>MGRDPNSTDNIRPTYQTDANGTYPTNSWQVTGQQNVINQRGGDQVSGWDNNTIWNGDATDTTNSYLKFGDPNNPDYQIRKYAKETNTPGLYDVYLNVKGNKQQNVKPVDIVLVVDMSGSMESNRWGTNRAGAVRTGVKNFLTSIQNAGLGNYVNVGLIGFSSPGYIGGKSGYISVKLGKAGNASQQQAINGALSPRFQGGTYTQIGLRQGSAMLNADTSGNKKMMILLTDGVPTFSNEVINSEWINGTLYGTNFGSSRDEPGNTARLRWPYTDSSGHYIYDTWPATLGEAKIAKDSGNEVHALGIQLADDDHYMTKEKIRQNMQLITNSPDLYEDADSADAVEAYLNNQAKDIIKNFNTVTDGTITDPIGTQFQYANNQATVTSVGKQTVPASELPSAAIQDGQLTVNHMNLGQDQEVQIHYQVRIKTEDAGFKPDFWYQMNGETLLTPKAGAAAVDFGIPSGRAPATTVYVQKQWRQLSNQSLPDTLNVTVQRKVADGSLDPNWQQTLVLKKADNWKASFTAPAYNNQGQSFSYVVKSEDASGIDLSSFISSQNMDQQTATLTLTNQQYGFQFQKKTTDGTDLSADQLKAMQFNLTQYSDNSFQQASKTNAITST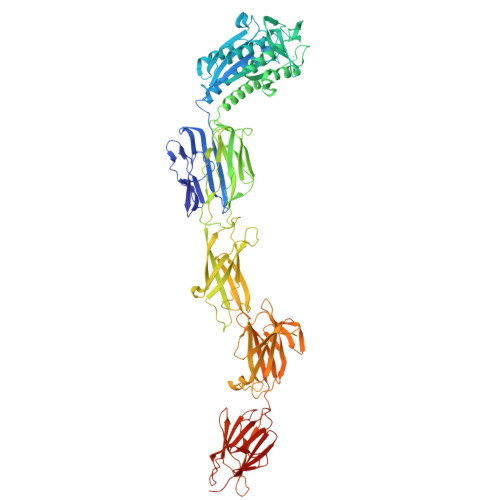DLQALAPGYYGIQEAAAPTGYQLDGTTYLFQLTSDGQWQYHGTKDNVTSGSVINGQQTLNPVGDKSDDFTVTGDHQQILTLTKYDEPKPSMTLRVIKQDNQSQYLAGAAFTLQPSAGEAETITSSATSEGQAFATKLVADGTYTMSETKAPDGYQSNPAKIAIQVATTGKEATVTIDGEALKPGESKNGYTLAIDGSTITLQAINQPLAILPLEHHHHHH[2x]> TLHDKQIRICHLFEQLSSATVIGDGDKHKHSDRLKNVGKLQPGAIFSCFHPDHLEEARHLYEVFWEAGDFNDFIEIAKEARTFVNEGLFAFAAEVAVLHRDDCKGLYVPPVQEIFPDKFIPSAAINEAFKKAHVRPEFDESPILVDVQDTGNILDPEYRLAYYREDVGINAHHWHWHLVYPSTWNPKYFGKKKDRKGELFYYMHQQMCARYDCERLSNGMHRMLPFNNFDEPLAGYAPHLTHVASGKYYSPRPDGLKLRDLGDIEISEMVRMRERILDSIHLGYVISEDGSHKTLDELHGTDILGALVESSYESVNHEYYGNLHNWGHVTMARIHDPDGRFHEEPGVMSDT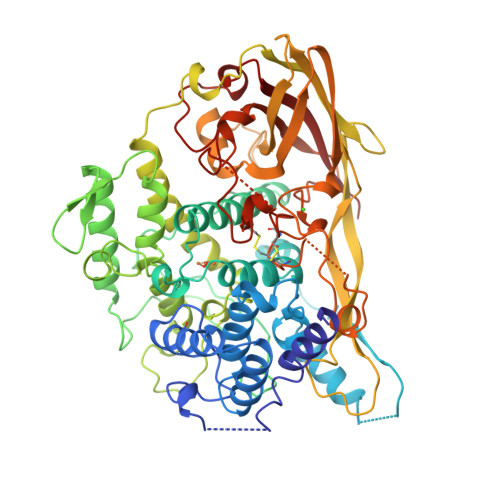STSLRDPIFYNWHRFIDNIFHEYKNTLKPYDHDVLNFPDIQVQDVTLHARVDNVVHTFMREQELELKHGINPGNARSIKARYYHLDHEPFSYAVNVQNNSASDKHATVRIFLAPKYDELGNEIKADELRRTAIELDKFKTDLHPGKNTVVRHSLDSSVTLSHQPTFEDLLHGVGLNEHKSEYCSCGWPSHLLVPKGNIKGMEYHLFVMLTDWDKDKVDGSESVACVDAVSYCGARDHKYPDKKPMGFPFDRPIHTEHISDFLTNNMFIKDIKIKFHE> AGGQQSFDLLVIGGGSGGLACAKEAAQLGKKVAVADYVEPSPRGTKWGLGGTCVNVGCIPKKLMHQAALLGGMIRDAHHYGWEVAQPVQHNWKTMAEAVQNHVKSLNWGHRVQLQDRKVKYFNIKASFVDEHTVRGVDKGGKATLLSAEHIVIATGGRPRYPTQVKGALEYGITSDDIFWLKESPGKTLVVGASYVALECAGFLTGIGLDTTVMMRSIPLRGFDQQMSSLVTEHMESHGTQFLKGCVPSHIKKLPTNQLQVTWEDHASGKEDTGTFDTVLWAIGRVPETRTLNLEKAGISTNPKNQKIIVDAQEATSVPHIYAIGDVAEGRPELTPTAIKAGKLLAQRLFGKSSTLMDYSNVPTTVFTPLEYGCVGLSEEEAVALHGQEHVEVYHAYYKPLEFTVADRDASQCYIKMVCMREPPQLVLGLHFLGPNAGEVTQGFALGIKCGASYAQVMQTVGIHPTC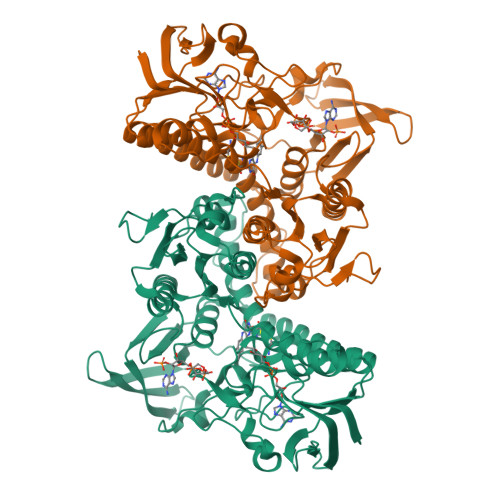SEEVVKLHISKRSGLEPTVTG> GAVQNDEVAAFCQSIMKLKTKFPYTDHCTNPGYLLSPVTVQRNMCGENASVKVSIEIEGLQLPVTFTCDVSSTVEIIIMQALCWVHDDLNQVDVGSYILKVCGQEEVLQNNHCLGSHEHIQNCRKWDTEIKLQLLTLSAMCQNLARTAEDDEAPVDLNGSGSVMTRHSAGAGSGASTGCPRGSRNIKEAWTATEQLQFTVYAAHGISSNWVSNYEKYYLICSLSHNGKDLFKPIQSKKVGTYKNAAYLIKWDELIIFPIQISQLPLESVLHLTLFGVLNQSSGSSPDSNKQRKGPEALGKVSLTLFDFKRFLTCGTKLAYLWTSSHTNSIPGAIPKKSYVMERIVLQVDFPSPAFDIIYTSPQIDRNIIQQDKLETLESDIKGKLLDIIHRDSSFGLSKEDKVFLWENRYYCLKHPNCLPKILASAPNWKWANLAKTYSLLHQWPPLCPLAALELLDAKFADQEVRSLAVSWMEAISDDELADLLPQFVQALKYEIYLNSSLVRFLLSRALGNIQIAHSLYWLLKDALHDTHFGSRYEHVLGALLSVGGKGLREELSKQMKLVQLLGGVAEKVRQASGSTRQVVLQKSMERVQSFFLRNKCRLPLKPSLVAKELNIKSCSFFSSNAMPLKV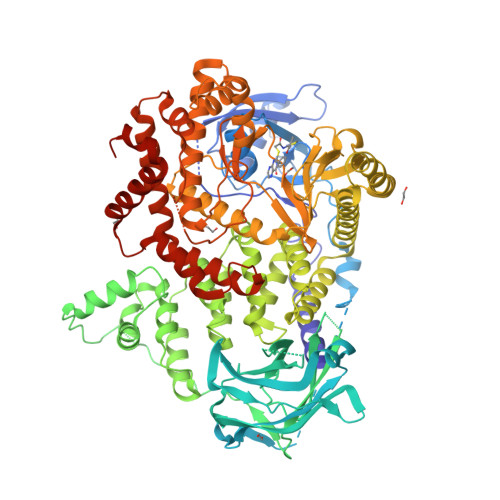TMVNADPLGEEINVMFKVGEDLRQDMLALQMIKIMDKIWLKEGLDLRMVIFRCLSTGRDRGMVELVPASDTLRKIQVEYGVTGSFKDKPLAEWLRKYNPSEEEYEKASENFIYSCAGCCVATYVLGICDRHNDNIMLRSTGHMFHIDFGKFLGHAQMFGSFKRDRAPFVLTSDMAYVINGGEKPTIRFQLFVDLCCQAYNLIRKQTNLFLNLLSLMIPSGLPELTSIQDLKYVRDALQPQTTDAEATIFFTRLIESSLGSIATKFNFFIHNLAQLRFSG>GAMKNSFDRLIDGLAKDYGMPGFPEKKHEHEVYCFEFKEVSIRIYQDKFKWVYFLSDIGVIDNLDSN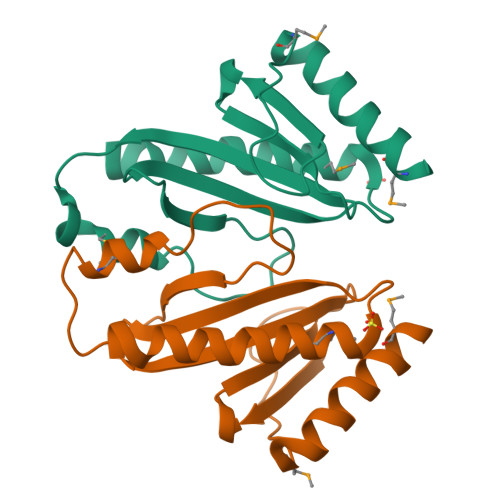ACQSLLRLNEFNLRTPFFTVGLNEKKDGVVHTRIPLLNLDNVEMRRVFEALLNLSGEVKKTFGFV[4x]>[2x]MPNTAMKKKVLLMGKSGSGKTSMRSIIFANYIARDTRRLGATIDVEHSHVRFLGNLVLNLWDCGGLDTFMENYFTSQRDNIFRNVEVLIYVFDVESRELEKDMHYYQSCLEAILQNSPDAKIFCLVHKMDLVQEDQRDLIFKEREEDLRRLSRPLECACFRTSIWDETLYKAWSSIVYQLIPNVQQLEMNLRNFAQIIEADEVLLFERATFLVISHYQCKEQRDVHRFEKISNIIKQFKLSCSKLAASFQSMEVRNSNFAAFIDIFTSNTYVMVVMSDPSIPSAATLINIRNARKHFEKLERVDGPKHSLLMR;>[2x]MSLQYGAEETPLAGSYGAADSFPKDFGYGVEEEEEE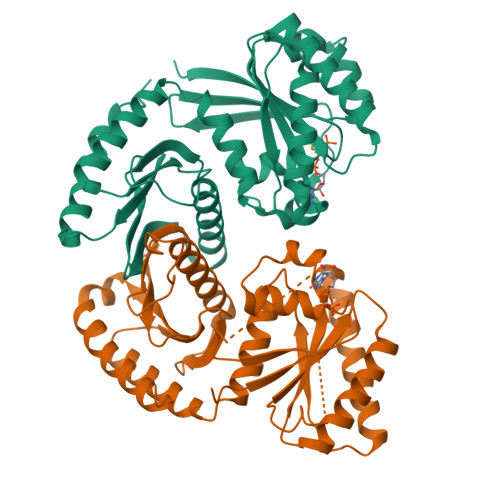AAAAGGGVGAGAGGGCGPGGADSSKPRILLMGLRRSGKNSIQKVVFHKMSPNETLFLESTNKIYKDDISNSSFVNFQIWDFPGQMDFFDPTFDYEMIFRGTGALIYVIDAQDDYMEALTRLHITVSKAYKVNPDMNFEVFIHKVDGLSDDHKIETQRDIHQRANDDLADAGLEKLHLSFYLTSIYDHSIFEAFSKVVQKLIPQLPTLENLLNIFISNSGIEKAFLFDVVSKIYIATDSSPVDMQSYELCCDMIDVVIDVSCIYGLKEDGSGSAYDKESMAIIKLNNTTVLYLKEVTKFLALVCILREESFERKGLIDYNFHCFRKAIHEVFEVGVTSHRSCGHQTSASSLKALTHNGTPRNAI>MSQVTDMRSNSQGLSLTDSVYERLLSERIIFLGSEVNDEIANRLCAQILLLAAEDASKDISLYINSPGGSISAGMAIYDTMVLAPCDIATYAMGMAASMGEFLLAAGTKGKRYALPHARILMHQPLGGVTGSAADIAIQAEQFAVIKKEMFRLNAEFTGQPIERIEADSDRDRWFTAAEALEYGFVDHIITRAHVNGEAQ[7x];>MNSQNSQIQPQARYILPSFIEHSSFGVKESNPYNKLFEERIIFLGVQVDDASANDIMAQLLVLESLDPDRDITMYINSPGGGFTSLMAIYDTMQYVRADIQTVCLGQAASAAAVLLAAGTPGKRMALPNARVLIHQPSLSGVIQGQFSDLE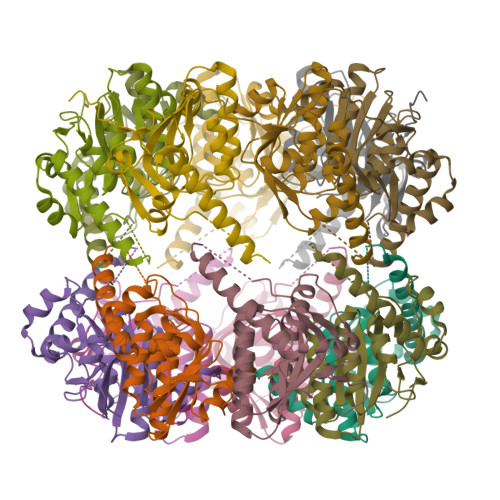IQAAEIERMRTLMETTLARHTGKDAGVIRKDTDRDKILTAEEAKDYGIIDTVLEYRKLSAQTA[7x]> PQPRKKRPEDFKFGKILGEGSFSTVVLARELATSREYAIKILEKRHIIKENKVPYVTRERDVMSRLDHPFFVKLYFTFQDDEKLYFGLSYAKNGELLKYIRKIGSFDETCTRFYTAEIVSALEYLHGKGIIHRDLKPENILLNEDMHIQITDFGTAKVLSPESKQARANSFVGTAQYVSPELLTEKSACKSSDLWA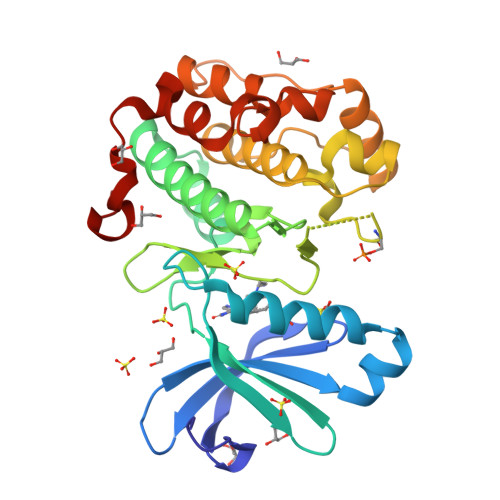LGCIIYQLVAGLPPFRAGNEYLIFQKIIKLEYDFPEKFFPKARDLVEKLLVLDATKRLGCEEMEGYGPLKAHPFFESVTWENLHQQTPPK>[2x]GPMTDWPVYHRIDGPIVMIGFGSIGRGTLPLIERHFAFDRSKLVVIDPSDEARKLAEARGVRFIQQAVTRDNYRELLVPLLTAGPGQGFCVNLSVDTSSLDIMELARENGALYIDTVVEPWLGFYFDPDLKPEARSNYALRETVLAARRNKPGGTTAVSCCGANPGMVSWFVKQALVNLAADLGVTGEEPTTREEWARLAMDLGVKGIHIAERDTQRASFPKPFDVFVNTWSVEGFVSEGLQPAELGWGTFERWMPDNARGHDSGCGAGIYLLQPGANTRVRSWTPTAMAQYGFLVTHNESISIADFLTVRDAAGQAVYRPTCHYAYHPCNDAVLSLHEMFGSGKRQSDWRILDETEIVDGIDELGVLLYGHGKNAYWYGSQLSIEETRRIAPDQNATGLQVSSAVLAGMVWALENPNAGIVEADDLDFRRCLEVQTPYLGPVVGVYTDWTPLAGRPGLFPEDIDTSDPWQFRNVLVRD

In contrast to its eukaryotic counterparts, bacterial HSS synthesizes 1 mol HSP from 2 mol PUT. NAD+ serves as a non-covalently bound prosthetic group for BvHSS. The interface area of the dimer was calculated as approximately 1700 Å2 by PDBsum indicating a stable dimer23. The BvHSS subunit consists of two domains as determined by CATH24: one “NAD(P)-binding Rossmann-like” domain (domain 1, residues 3–163 and 394–425) and one “homospermidine-synthase-like domain” (domain 2, residues 164–395 and 426–477) as shown in Fig. 2a and S1. The crystal structures of BvHSS containing NAD+ clearly show that the active site is localized inside each subunit.

The electron density at the active site of subunit B is interpreted as a hydride transfer from PUT carbon C4 to NAD+ carbon C4N representing a “transition-close” state of the oxidation at carbon C4. The electron density at the active site of subunit A is interpreted as representing the hydride transfer from carbon C4N of NADH to the still oxidized carbon C05 of HSP, with a partial double bond between carbon C05 and nitrogen N06 of HSP representing a partial Schiff base (see subsection “Hypothesis of the Reaction Steps of BvHSS Catalysis” for details). The inner most amino group at nitrogen N01 of HSP or nitrogen N1 of PUT is coordinated to residues Glu-210 and Asn-162 (inner amino site), whereas the amino group at nitrogen N11 of HSP is coordinated to Glu-237 and oxygen O2D of NADH (outer amino site). The nitrogen N2 of PUT is coordinated to Asn-162 (center amino site). The polyamine nitrogens (N2 of PUT, N06 of HSP) are bound with a non-optimal off-center geometry relative to the center of the 6-membered (benzene) ring of the respective Trp-229 side chain. Based on calculated interaction energies of benzene with NH4+32, these positions will most likely result in interaction energies significantly contributing to substrate binding and recognition via cation-π interaction. The substrates are further stabilized by hydrophobic interactions with Val-115, Pro-163, Trp-229, His-296, Tyr-323, Tyr-325, and Thr-396. The binding position between the inner amino site and center amino site will be referred to as the inner (binding) site, whereas the binding position between the center amino site and outer amino site will be referred to as the outer (binding) site. In accordance with the observed electron density distribution of substrate bound BvHSS, a hydride transition state with a partially aromatic nicotine amid ring and a positive partial charge at PUT carbon C4 seems probable. Thus, DAP can compete against PUT for both binding sites explaining its reported competitive inhibitory effect. The aforementioned HSS products and the observed diamine binding patterns imply a highly specific PUT binding site at the inner site discriminating, via carbon chain length, at which position the redox reaction solely can take place.>[3x]MTDQVFGKVSKVVCVGAGYVGGPTCAMIAHKCPHITVTVVDMNTAKIAEWNSDKLPIYEPGLDEIVFAARGRNLFFSSDIPKAIAEADLIFISVNTPTKMYGRG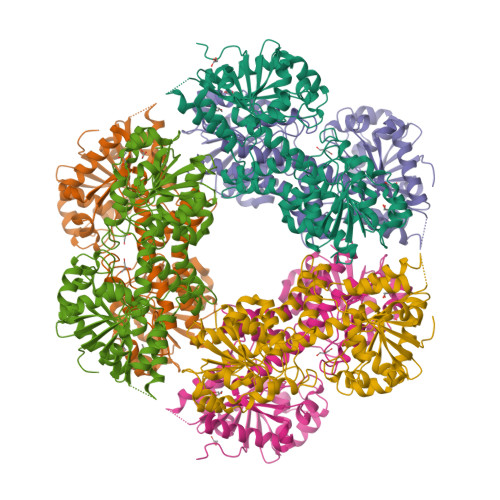KGMAPDLKYVESVSRTIAQYAGGPKIVVEKSTVPVKAAESIGCILREAQKNNENLKFQVLSNPEFLAEGTAMKDLANPDRVLIGGESSPEGLQAVAELVRIYENWVPRNRIITTNTWSSELSKLVANAFLAQRISSINSISAVCEATGAEISEVAHAVGYDTRIGSKFLQASVGFGGSCFQKDVLSLVYLCESLNLPQVADYWQGVININNWQRRRFADKIIAELFNTVTDKKIAIFGFAFKKNTGDTRESSAIHVIKHLMEEHAKLSVYDPKVQKSQMLNDLASVTSAQDVERLITVESDPYAAARGAHAIVVLTEWDEFVELNYSQIHNDMQHPAAIFDGRLILDQKALREIGFRTFAIGTSPDQAYNLFGTAGY(3S)-3-[({(2S)-5-[(N-ACETYL-L-ALPHA-ASPARTYL)AMINO]-4-OXO-1,2,4,5,6,7-HEXAHYDROAZEPINO[3,2,1-HI]INDOL-2-YL}CARBONYL)AMINO]-5-(BENZYLSULFANYL)-4-OXOPENTANOIC 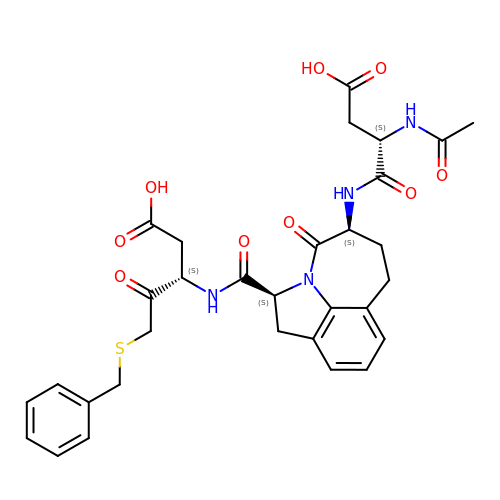ACID | C31 H34 N4 O9 S | PEECWFLPGAWBQR-ZJZGAYNASA-N>MASKIFQYNQHKQETNETLNHHNCSNMQRAFNLKEEMLTNKSIDCRPSNETLEYIKGEQHDRWDSKTKTVLDSSRDTGRGVKYWFCYSTKCYYFIMNKTTWSGCKANCQHYGVPILKIEDEDELKFLQRHVIPGNYWIGLSYDKKKKEWAWIDNGPSKLDMKIKKMNFKSRGCVFLSKARIEDIDCNIPYYCICGKKLDKFP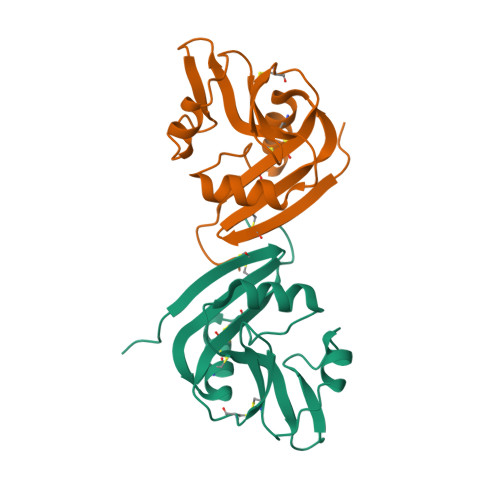D[4x]>[2x]MSFKPTISVHATPQELSAAGCRKIVEIIEASGSQQWPLSIALAGGSTPKMTYARLHDEHLNLLREKRALRFFMGDERMVPADSTDSNYNMAREVLLHDIPDDLVFPFDTSAVTPSAEATSADAMRVAEAYGKQLASLLPLKSVGEAGPKVPVFDVVLLGLGSDGHTASIFPGSQAEKETDGKVVVSVGFPSETMKPKVWRVTLSPATIMQARNVIVLATGA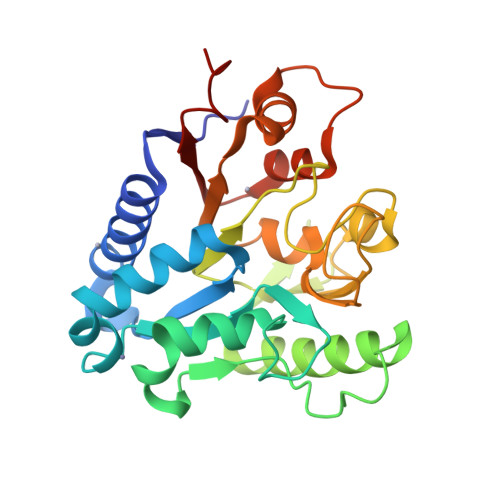EKKWVVDGILADTAHKAPVARFLRGCEGNVSFLLDKEIAENLAKF> MAN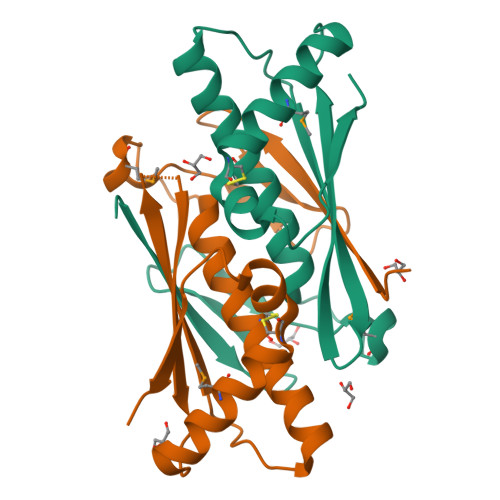VYTAEATATGGRAGTTRSSDDRLNLDLSVPAEMGGDGGPGTNPEQLFAAGYAACFQGALGVVSRRQKIDVPADSTITARVGLQKAGLAFALDVELEGHFPGLSREQAEGLMHAAHEVCPYSAATRNNVDVRLKVRE;> MANVYTAEATATGGRAGTTRSSDDRLNLDLSVPAEMGGDGGPGTNPEQLFAAGYAACFQGALGVVSRRNKIDVPADSTITARVGLQKAGLAFALDVELEGHFPGLSREQAEGLMHAAHEVCPYSAATRNNVDVRLKVRE>[2x]MKSSNRSENIRVGTENTVGKSKSVTVIGLGPMGKAMAAAFLEHGYKVTVWNRTSNKADELITKGAVRASTVHEALAANELVILSLTDYDAMYTILEPASENLSGKVLVNLSSDTPDKAREA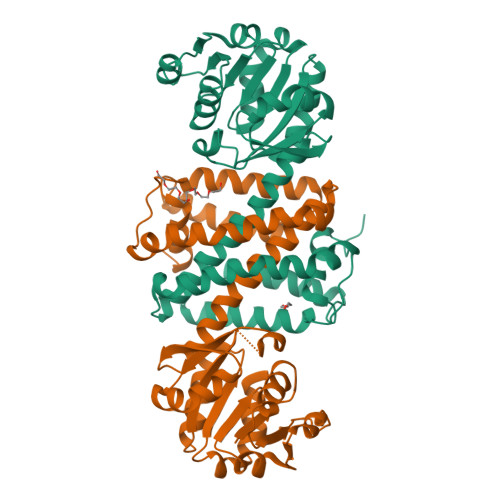AKWLANRGAGHITGGVQVPPSGIGKPESSTYYSGPKEVFEANKETLEVLTGTDYRGEDPGLAALYYQIQMDMFWTAMLSYLHATAVAQANGITAEQFLPYAAETMSSLPKFIEFYTPRINAGEYPGDVDRLAMGMASVEHVVHTTQDAGIDITLPTAVLEVFRRGMENGHAGNSFTSLIEIFKKSDIRP> AAPGKPTIAWGNTKFAIVEVDQAATAYNNLVKVKNAADVSVSWNLWNGDTGTTAKVLLNGKEAWSGPSTGSSGTANFKVNKGGRYQMQVALCNADGCTASDATEIVVADTDGSHLAPLKEPLLEKNKPYKQNSGKVVGSYFVEWGVYGRNFTVDKIPAQNLTHLLYGFIPICGGNGINDSLKE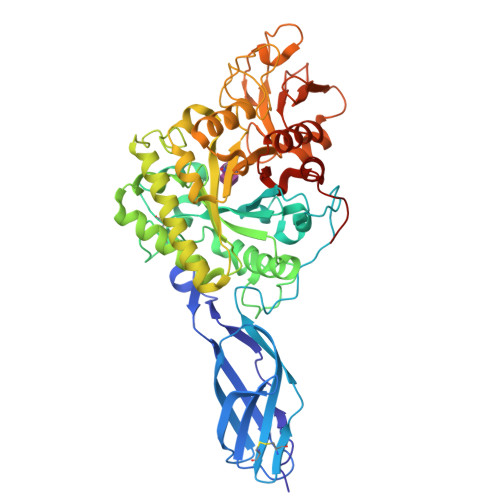IEGSFQALQRSCQGREDFKVSIHDPFAALQKAQKGVTAWDDPYKGNFGQLMALKQAHPDLKILPSIGGWTLSDPFFFMGDKVKRDRFVGSVKEFLQTWKFFDGVDIDWEFPGGKGANPNLGSPQDGETYVLLMKELRAMLDQLSVETGRKYELTSAISAGKDKIDKVAYNVAQNSMDHIFLMSYDFYGAFDLKNLGHQTALNAPAWKPDTAYTTVNGVNALLAQGVKPGKIVVGTAMYGRGWTGVNGYQNNIPFTGTATGPVKGTWENGIVDYRQIAGQFMSGEWQYTYDATAEAPYVFKPSTGDLITFDDARSVQAKGKYVLDKQLGGLFSWEIDADNGDILNSMNASLGNSAGVQ> GPLGSMDPSVKKDEIYYTILNIIQNYFIEYCTGKNRNFHVEDENTYIIVKNMCDIILRDNIVEFRKDIDRCSDIENEIPEIVYDTIHDKITWGRVISIIAFGAYVTKVFKEKGRDNVVDLMPDIITESLLSRCRSWLSDQN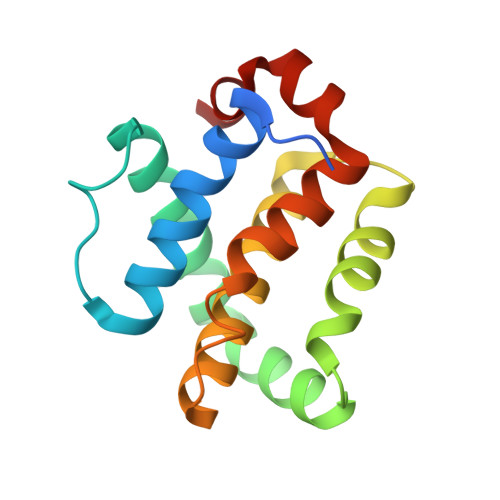CWDGLKA> MAPFRQDSILIIYPRSQTTLVQFGLNEETFTVPELEIPTQIYRTTRQDGSYTYHSTNKDNKAELIKPIQNGEIIDISAFTQFLRLIFVSILSDRANKNQDAFEAELSNIPLLLITHHSW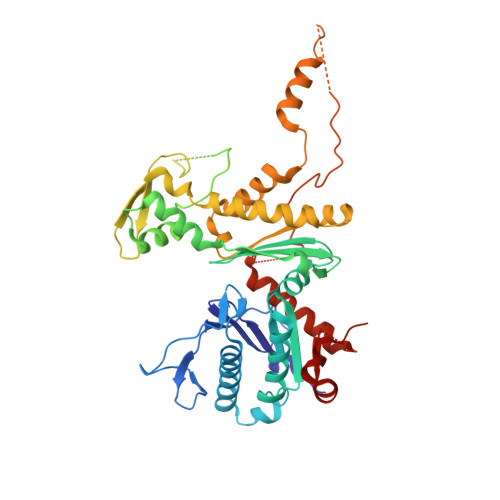SQSDLEIITQYVFESLEINNLIQLPASLAATYSMISLQNCCIIDVGTHHTDIIPIVDYAQLDHLVSSIPMGGQSINDSLKKLLPQWDDDQIESLKKSPIFEVLSDDAKKLSSFDFGNENEDEDEGTLNVAEIITSGRDTREVLEERERGQKVKNVKNSDLEFNTFWDEKGNEIKVGKQRFQGCNNLIKNISNRVGLTLDNIDDINKAKAVWENIIIVGGTTSISGFKEALLGQLLKDHLIIEPEEEKSKREEEAKSVLPAATKKKSKFMTNSTAFVPTIEYVQCPTVIKLAKYPDYFPEWKKSGYSEIIFLGAQIVSKQIFTHPKDTFYITREKYNMKGPAALWDVQF> GAMSSKNEWRKSAIANTLLYLRLKNIYVSADDFVEEQNVYVLPKNLLKKFIEISDVK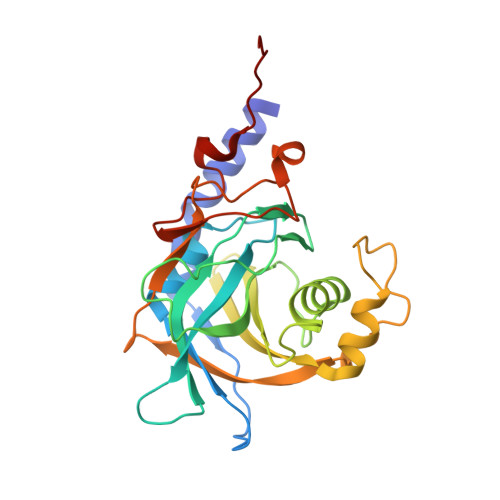IQVAAFIYGMSAKDHPKVKEIKTVVLVPQLGHVGSVQISNIPDIGDLPDTEGLELLGWIHTQTEELKFMAASEVATHSKLFADKKRDCIDISIFSTPGSVSLSAYNLTDEGYQWGEENKDIMNVLSEGFEPTFSTHAQLLLSDRITGNFIIPSGNVWNYTFMGTAFNQEGDYNFKYGIPLEFYNEMHRPVHFLQFSE> MHHHHHHHDGTEDPIHDRTSDYHKYLKVKQGDSDLFKLTVSDKRYIWYNPDPKERDSYECGEIVSETSDSFTFKTVDGQDRQVKKDDANQRNPIKFDGVEDMSELSYLNEPAVFHNLRVRYNQDLIYTYSGLFLVAVNPFKRIPIYTQEMVDIFKGRRRNEVAPHIFAISDVAYRSMLDDRQNQSLLITGESGAGKTENTKKVIQYLASVAGRNQANGSGVLEQQILQANPILEAFGNAKTTRNNNSSRFGKFIEIQFNSAGFISGASIQSYLLEKSRVVFQSETERNYHIFYQLLAGATAEEKKALHLAGPESFNYLNQSGCVDIKGVSDSEEFKITRQAMDIVGFSQEEQMSIFKIIAGILHLGNIKFEKGAGEGAVLKDKTALNAASTVFGVNPSVLEKALMEPRILAGRDLVAQHLNVEKSSSSRDALVKALYGRLFLWLVKKINNVLCQERKAYFIGVLDISGFEIFKVNSFEQLCINYTNEKLQQFFNHHMFKLEQEEYLK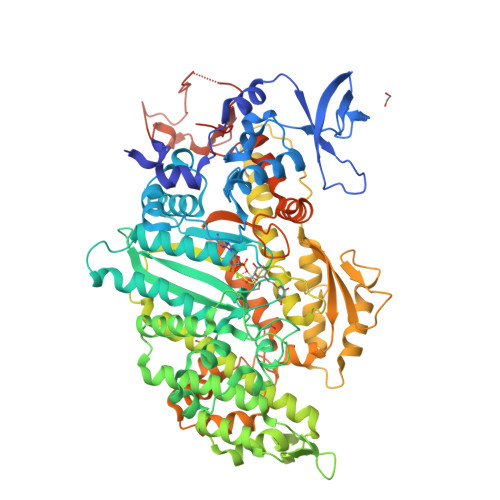EKINWTFIDFGLDSQATIDLIDGRQPPGILALLDEQSVFPNATDNTLITKLHSHFSKKNAKYEEPRFSKTEFGVTHYAGQVMYEIQDWLEKNKDPLQQDLELCFKDSSDNVVTKLFNDPNIASRAKKGANFITVAAQYKEQLASLMATLETTNPHFVRCIIPNNKQLPAKLEDKVVLDQLRCNGVLEGIRITRKGFPNRIIYADFVKRYYLLAPNVPRDAEDSQKATDAVLKHLNIDPEQYRFGITKIFFRAGQLARIEEAREQRLESNEPPMDFDDDIPF>ISSQAVTSVPYKWDNVVIGGGGGFMPGIVFNETEKDLIYARAAIGGAYRWDPSTETWIPLLDHFQMDEYSYYGVESIATDPVDPNRVYIVAGMYTNDWLPNMGAILRSTDRGETWEKTILPFKMGGNMPGRSMGERLAIDPNDNRILYLGTRCGNGLWRSTDYGVTWSKVESFPNPGTYIYDPNFDYTKDIIGVVWVVFDKSSSTPGNPTKTIYVGVADKNESIYRSTDGGVTWKAVPGQPKGLLPHHGVLASNGMLYITYGDTCGPYDGNGKGQVWKFNTRTGEWIDITPIPYSSSDNRFCFAGLAVDRQNPDIIMVTSMNAWWPDEYIFRSTDGGATWKNIWEWGMYPERILHYEIDISAAPWLDWGTEKQLPEINPKLGWMIGDIEIDPFNSDRMMYVTGATIYGCDNLTDWDRGGKVKIEVKATGIEECAVLDLVSPPEGAPLVSAVGDLVGFVHDDLKVGPKKMHVPSYSSGTGIDYAELVPNFMALVAKADLYDVKKISFSYDGGRNWFQPPNEAPNSVGGGSVAVAADAKSVIWTPENASPAVT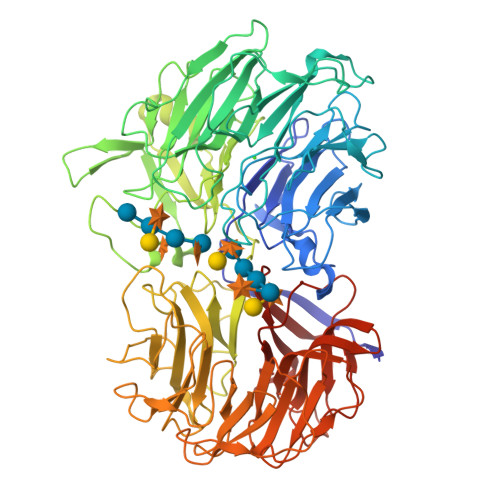TDNGNSWKVCTNLGMGAVVASDRVNGKKFYAFYNGKFYISTDGGLTFTDTKAPQLPKSVNKIKAVPGKEGHVWLAAREGGLWRSTDGGYTFEKLSNVDTAHVVGFGKAAPGQDYMAIYITGKIDNVLGFFRSDDAGKTWVRINDDEHGYGAVDTAITGDPRVYGRVYIATNGRGIVYGEPASDEPV[2x]> MTSQIQK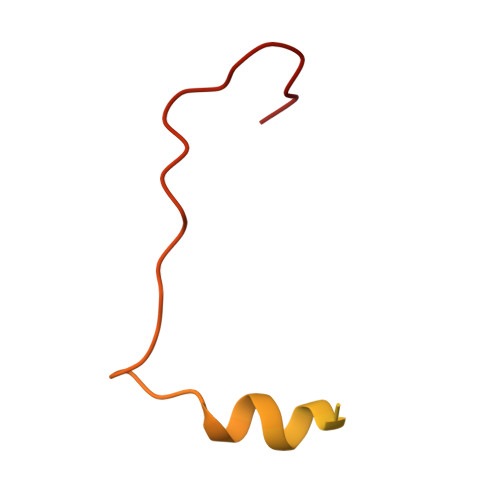WGNSLALRIPKALAQQVGLTQSSEVELLLQDGQIVIRPVPARQYDLAALLAEMTPENLHGETDWGALEGREEW>[5x]MEAIKGSDVNVPDAVFAWMLDGRGGVKPLENTDVIDEAHPCWLHLNYVHHDSAQWLATTPLLPNNVRDALAGESTRPRVSRLGEGTLITLRCINGSTDERPDQLVAMRVYMDGRLIVSTRQR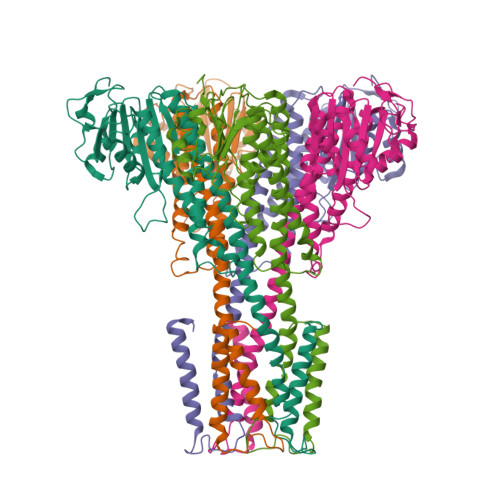KVLALDDVVSDLEEGTGPTDCGGWLVDVCDALTDHSSEFIEQLHDKIIDLEDNLLDQQIPPRGFLALLRKQLIVMRRYMAPQRDVYARLASERLPWMSDDQRRRMQDIADRLGRGLDEIDACIARTGVMADEIAQVMQENLARRTYTMSLMAMVFLPSTFLTGLFGVNLGGIPGGGWQFGFSIFCILLVVLIGGVALWLHRSKWL>GGTDRMARLLGELLVSTDDSGNLAVLRTPPGAAHYLASAIDRAALPQVVGTIAGDDTILVVAREPTTGAQLAGMFENLR[6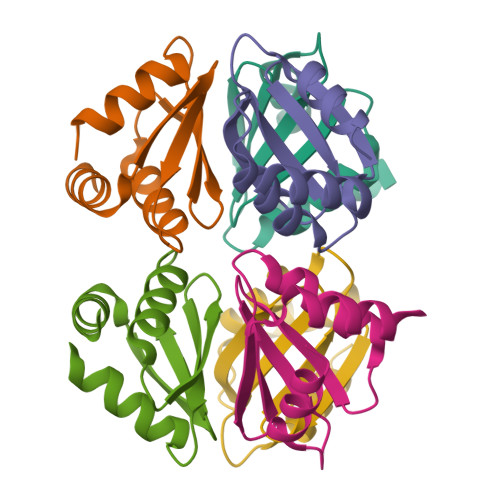x]> QQIGTLTTETHPPLTWQTCTSGGSCTTNNGKVVLDANWRWLHSTSGSTNCYTGNTWNTTLCPDDTTCAQNCALDGADYEGTYGITASGNSLRLNFVTNGSQKNVGSRTYLMKDDTHYQTFNLLNQEFTFDVDVSGLPCGLNGALYMVPMAADGGVSNEPNNKAGAQYGVGYCDSQCPRDLKFIAGSANVQGWEPASNSANSGLGGNGSCCAELDIWEANSISAALTPHSADTVTQTVCNGDDCGGTYSNDRYSGTTDPDGCDFNSYRQGDTSFYGPGKTVDTNSKFTVVTQFLT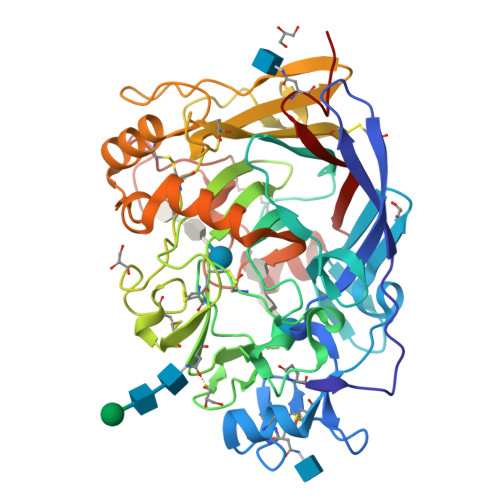DSSGNLNEIKRFYVQNGVVIPNSQSTIAGISGNSITQDYCTAQKQVFGDTNTWEDHGGFQSMTNAFKAGMVLVMSLWDDYYADMLWLDSVAYPTDADPSTPGVARGTCSTTSGVPSDIESSAASAYVIYSNIKVGPINSTFSGT>[12x]MGIISYVKK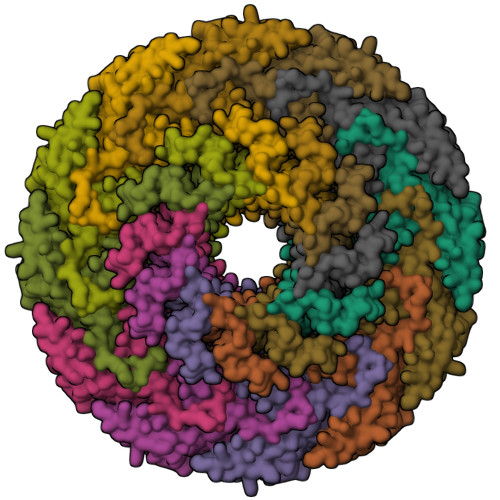LFKRPAGEIMRMSSGNIGVYKLDDSRVDYELARELYQNKNANYKLGSSFVRPIVNSTTGFMGVPHFQIEDEEAQYILDEFVLDNTSKMLKTHTDSLKQGDCYIWITREERENPLYPDKKVRLIYNFISPEEVKEIILDPTTKEPIAYILESQNEWTDLGENKRKAKVKQIITAESRFVEVEGDKIEGLEEGETPNVWGFIPIIHFKNEADETLKYGQSDIEPIEPLLKAYHDVMLHALKGSKMHSTPKLKLKLTDVASFLAHNFGVEDPVKFAKEGGKINLDGHEILFLNKDEEAEFVEVKSAIGDAKELLKLLFYCIVDVSETPEFIFGVHTPSALASVKEQMPIMVNKIRRKREQFTNSWQLLARMVLIMSSNSSGMKYSSYDVTIGWDEVNPRDDKELAETLEKVCCALDKALEGGFISEESTVNFLAQYIDTMSNYISDDPEREGEREKIIKTKMLKYRLDDSQGLNDESNEIEKEINKIKDNNGNG> DISEPPLHDFYCSRLLDLVFLLDGSSRLSEAEFEVLKAFVVDMMERLRISQKWVRVAVVEYHDGSHAYIGLKDRKRPSELRRIASQVKYAGSQVASTSEVLKYTLFQIFSKIDRPEASRIALLLMASQEPQRMSRNFV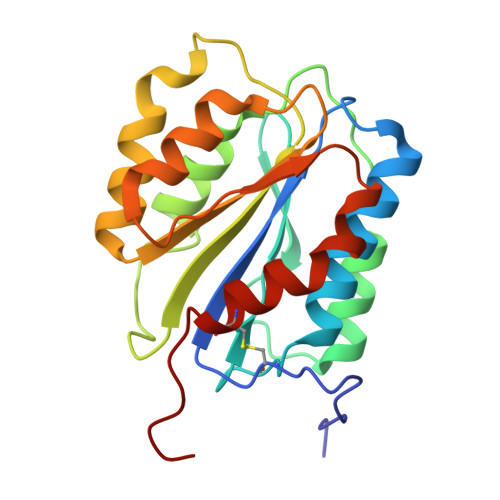RYVQGLKKKKVIVIPVGIGPHANLKQIRLIEKQAPENKAFVLSSVDELEQQRDEIVSYLCDLAPEAPPPT Holliday junction resolution is a crucial process in homologous recombination and DNA double-strand break repair. Holliday junction (HJ) is a four-way structured DNA intermediate formed during the homologous recombination. Canonical HJ resolvases introduce two symmetrical nicks across the junction center by functioning as homodimers, and exhibit strong structure- and sequence-specificities in HJ cleavage. The RNase H-like enzymes, including RuvC and MOC1, typically feature three or more conserved carboxylates, known as the DDE motif, in their active sites.

HJ cleavage was initiated by incubating the crystals in a solution supplemented with 10 mM Mn2+ ions for various periods. The first metal ion rapidly appeared within both active sites for approximately 15 s after soaking in Mn2+ ions. It aligns with the A-site of the two-metal-ion mechanism proposed by Steitz and Steitz30. The single Mn2+ is coordinated by the pro-Rp oxygen of scissile phosphate, the carboxylate groups of D115 and E257, along with water molecules, forming an irregular coordination geometry. In comparison to the ground state, the binding of Mn2+-A triggers a notable conformational change of E257, while the other residues mostly remain unchanged. The second Mn2+ emerged at the B-site by approximately 75 s. This sequential metal ion binding within the two sites might be attributed to the more solvent accessibility of the former compared to the latter.

>[2x]GWVIGVDPDIGGAIAVLSPDGSSQVFDNPFVHIVVSEVIRKRLDTKSIIQLLRGLDAPPGTTAYIEKSSPFPTDGKQGWWSTGFSYGLWIASLVASGFSVVPIASQTWKAYFGLMRSETPKDDSRQAASILFPDKDQSLKLKKHHGRAEALLLAAYGKGLVLP> MNLVLMGLPGAGKGTQAEKIVEKYGIPHISTGDMFRAAIKEGTELGLKAKSFMDKGELVPDEVTIGIVRERLSKDDCKKGFLLDGFPRTVAQAEALDNILKELGKK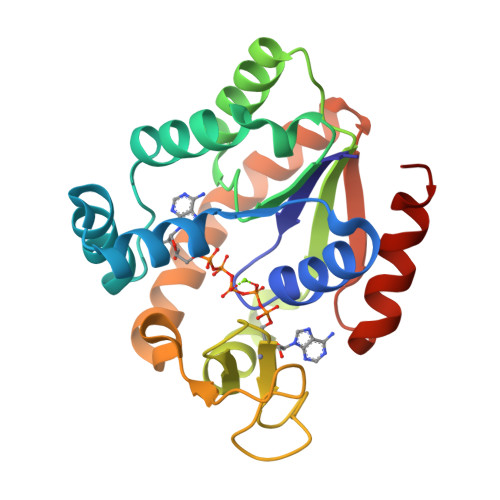LDYVINIEVPKEELMERLTGRRICKTCGATYHLIFNPPKVEGVCDKCGGELYQRADDNEETVANRLDVNMKQTQPLLDFYEEKGYLRNIDGQQDINKVFADIDALLGGLKQ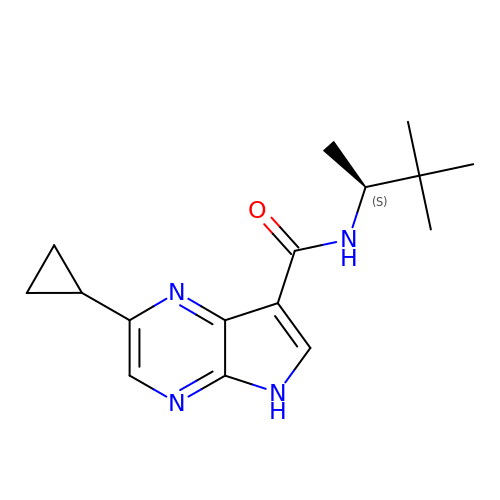2-cyclopropyl-N-[(2S)-3,3-dimethylbutan-2-yl]-5H-pyrrolo[2,3-b]pyrazine-7-carboxamide | C16 H22 N4 O | YCFLEMHGWPQDSP-VIFPVBQESA-N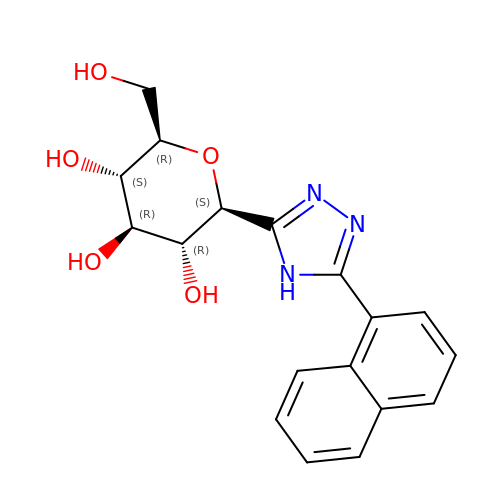(2~{R},3~{S},4~{R},5~{R},6~{S})-2-(hydroxymethyl)-6-(5-naphthalen-1-yl-4~{H}-1,2,4-triazol-3-yl)oxane-3,4,5-triol | C18 H19 N3 O5 | UGWCMNZLMGJTJS-IBEHDNSVSA-N GUANOSINE-2'-MONOPHOSPHATE | C10 H14 N5 O8 P | 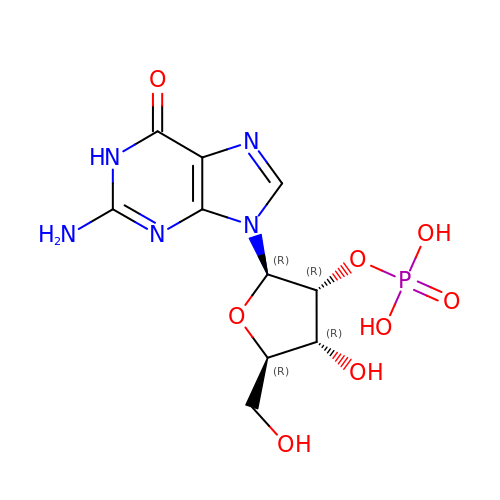WTIFIAZWCCBCGE-UUOKFMHZSA-N> FGSSHSTNDAKSPTLSESHKSARNVLENIGIKIYNQEIKKKNPYEQQLKGTLSRAQFVDALSSRYIEGRNSDGNSCNLDHLFHTNIKTGYNEGRKPCYGREQNRFDENAEAYCNSDKIRGNENNANGAACAPPRRRHICDQNLEFLDNKNTNTAHDLLGNVLVTAKYEGNYIVNDHPDKNSNGNKAGICTSLARSFADIGDIVRGRDMFLPNKDDKVQKGLQVVFKKIYKSLTPEARKHYAHGDGSGNYAKLREDWWTINREQIWKALTCSAPYYADYFRKGSDGTLHFSSHGKCGHNEGAPPTYLDYVPQFLRWFEEWSEEFCRIKKIKIDKVKKECRDEQNKKYCSGDGHDCTQTNLAHNQIFVDLDCPRCQDQCIKYNEWIVKKLEEFYKQNLKYSMEI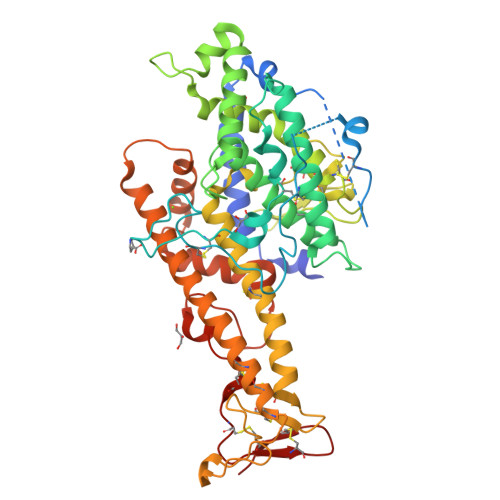QKWKKTKNNYYDKEFYENLDKKSYSTIDKFLNLLNNGKHCHDNKDEKNKIDFNKPIKTFSISEYCKTCPLYGVTCTNRGICIHNS(5S)-5-AMINO-3-OXO-HEXANOIC ACID | C6 H11 N O3 | 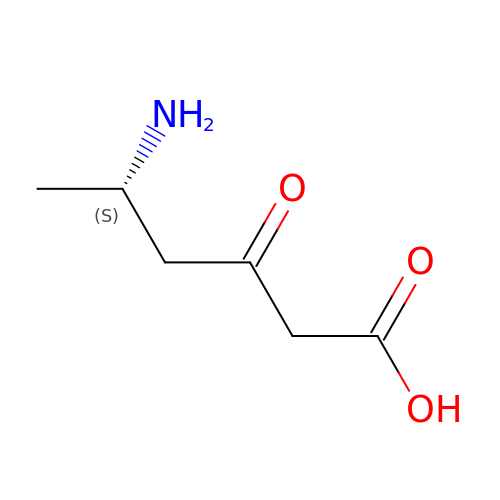FAASBXNEOGMQHS-BYPYZUCNSA-N Enhanced ABA levels elicited in response to drought are perceived by the PYR/PYL/RCAR family of ABA receptors and the clade A subfamily of protein phosphatases type 2C (PP2Cs), which act as necessary ABA co-receptors in ternary complexes. In the resting state, PYLR/PYL/RCAR receptors display an open ABA binding cavity flanked by two highly conserved loops, named as gate/CL2/β3-β4 loop and latch/CL3/β5-β6 loop. Specifically, both gate and latch loops define a surface that enables the receptor to dock into the PP2C active site. The formation of receptor-ABA-phosphatase complexes causes the dissociation of different PP2C-SnRK2 complexes and abolishes PP2C-mediated inhibition of the SnRK2s, triggering ABA response.

We reasoned that swapping the positions of the SO2 and CH2 moieties in the SB linker might contribute to fill this cavity by promoting the formation of a hydrogen bond between the SO2 moiety of the agonist and the Lys88 side chain, increasing ligand activity. We, therefore, synthesized two new compounds incorporating the above swap, iSB07 and iSB09 (“inverted SB”). Compared to iSB07, iSB09 contains a larger alkyl group (ethyl versus methyl) at the dihydroquinoline ring that might increase ligand activity through interaction with the 3′ tunnel for SB-01. To gain insight into the structural basis of iSB agonist activity, we solved the crystal structures of CsPYL1-iSB07-HAB1, CsPYL1-iSB09-HAB1, CsPYL15m-iSB07-HAB1, and CsPYL15m-iSB09-HAB1. Consistent with our docking predictions, both iSB07 and iSB09 complexes display the hydrogen bond network to conform the Trp lock and the compounds show a hydrogen bond between the oxygen of the SO2 moiety and side-chain NH3+ of Lys88 and, unexpectedly, an additional one to the guanidinium moiety of Arg108 side chain. In addition, iSB09 structures reveal that iSB09’s ethyl group, compared to iSB07’s methyl group, increases the number of hydrophobic contacts at the 3′ tunnel without distorting the conformation of the gate. The structural work provided the basis of such behavior, i.e., iSB07 and iSB09 sulfonamide linkers form additional H-bonds with respect to those observed in the SB complex. In particular, that formed between the oxygen of the SO2 moiety and the NH+ of Lys88 side-chain. In this work, we took advantage of structural knowledge on crop ABA receptors, docking studies, and structure-guided ligand optimization to generate iSB09. This synthetic compound displays a U-shaped conformation in the CsPYL1 binding pocket, which is shared with all sulfonamide-based agonist molecules.

> MNNNKAEADTSSSMADPETRPTYTTHHLAIPSGVTQDEFDELKQSVVEFHTYQLSQNQCSSLLAQRIRAPNDVVWSIVRRFDQPQTYKHFIKSCSVSDNFTMAVGSTRDVNVISGLPAATSTERLDILDDDRQVTGFSIIGGEHRLRNYRSVTSVHGFNRDGAICTVVLESYVVDVPEGNTEEDTRLFADTVVKLNLQKLVSVAESQVI;> RSVYELDCIPLWGVVSIQGNRSEMEDAFAVSPHFLKLPIKMLMGDHAGMSPSLTHLTGHFFGVYDGHGGHKVADYCRDRLHFALAEEIERIKDELCKRNTGEGRQVQWDKVFTSCFLTVDGEIEGKIGRAVVGSSDKVLEAVASETVGSTAVVALVCSSHIVVSNCGDSRAVLFRGKEAMPLSVDHKPDREDEYARIENAGGKVIQWQGARVFGVLAMSRSIGDRYLKPYVIPEPEVTFMPRSREDECLILASDGLWDVMNNQEVCEIARRRILMWHKKNGAPPLAERGKGIDPACQAAADYLSMLALQKGSKDNISIIVIDLKAQRKFKTRT> MFKKFDEKENVSNCIQLKTSVIKGIKNQLIEQFPGIEPWLNQIMPKKDPVKIVRCHEHIEILTVNGELLFFRQREGPFYPTLRLLHKYPFILPHQQVDKGAIKFVLSGANIMC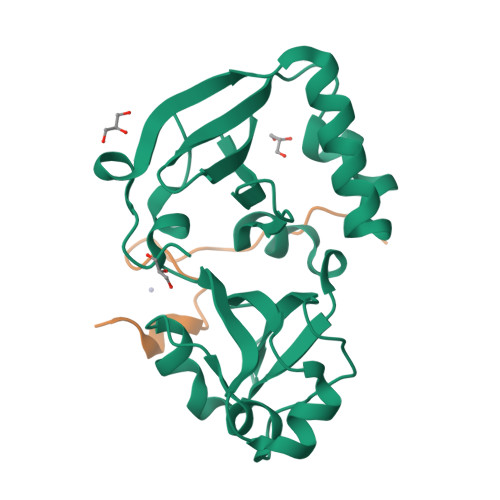PGLTSPGAKLYPAAVDTIVAIMAEGKQHALCVGVMKMSAEDIEKVNKGIGIENIHYLNDGLWHMKTYK;> MHHHHHHDADYPLRVLYCGVCSLPTEYCEYMPDVA The following permanent integration of this viral DNA by the viral-encoded integrase (IN) into the host chromosome is a necessary step in virus replication. In most retrovirus systems, IN first removes a dinucleotide from both termini of the linear blunt-ended viral DNA (∼10 kb), termed 3′ OH processing. Next, the same active sites catalyze the concerted transesterification reactions of the nascent 3′ OH groups into the cell DNA. RSV IN consists of the N-terminal domain (NTD) (residues 1–44), the catalytic core domain (CCD) (residues 50–214), and the C-terminal domain (CTD) (residues 222–286), similar in size to the corresponding domains of HIV IN.

In this report, we describe crystallographic analyses of a three-domain RSV IN as well as its CCD-CTD fragment in a new crystal form at a much improved resolution compared to previous studies. Although crystallization of a purified cross-linked IN-DNA complex has not been successful, we have been able to collect a 1.86 Å resolution dataset on a crystal of RSV IN(49–270) cross-linked in crystallo to a short viral DNA end substrate (5/7 hairpin DNA). The crystallized RSV IN (49–270) contained mutations S124D, C125A, E157C, and F199K. In our crystallographic model of RSV IN(49–270), the average atomic B-factors refined isotropically at 1.86 Å resolution for the CCD, CTD, and the inter-domain linker are 35.6 Å2, 47.9 Å2, and 30.7 Å2, respectively. As noted by Yang et al., the relative configuration between the CCDs and CTDs of RSV IN is stabilized by a large number of hydrogen bonds made by residues in or around the linker segment. Given the high similarity between all the crystal structures determined in different contexts, it seems likely that the observed conformation represents the intrinsically stable native conformation of the CCDs and CTDs, rather than an arbitral conformation captured by crystal lattice contacts. We have provided data rather contrary to this idea; a particular conformation of the CCD and CTD of RSV IN is observed independently of crystal contacts, and appears to be important for viral DNA binding. Our structural and mutation studies collectively suggested a role for the asymmetrically associated CTD dimer of RSV IN in viral DNA binding. The crystal structures, combined with earlier structural studies and our in vitro functional analyses, suggest that the asymmetric interaction between the two CTDs is an essential feature of an RSV IN dimer for viral DNA binding and catalysis, whereas the highly flexible NTD is required for IN tetramerization to promote concerted integration.

>GVNPRGLGPLQIWQTDFTLEPRMAPRSWLAVTVDTASSAIVVTQHGRVTSVAVQHHWATAIAVLGRPKAIKTDNGDAFTSKSTREWLARWGIAHTTGIPGNSQGQAMVCRANRLLKDKIRVLAEGDGFMKRIPTSKQGELLAKAMYALNHKERGENTKTPIQKHWRPTVLTEGPPVKIRIETGEWEKGWNVLVWGRGYAAVKNRDTDKVIWVPSRKVKPDIT[2x]6,11-DIHYDRO-11-ETHYL-6-METHYL-9-NITRO-5H-PYRIDO[2,3-B][1,5]BENZODIAZEPIN-5-ONE | C15 H14 N4 O3 | 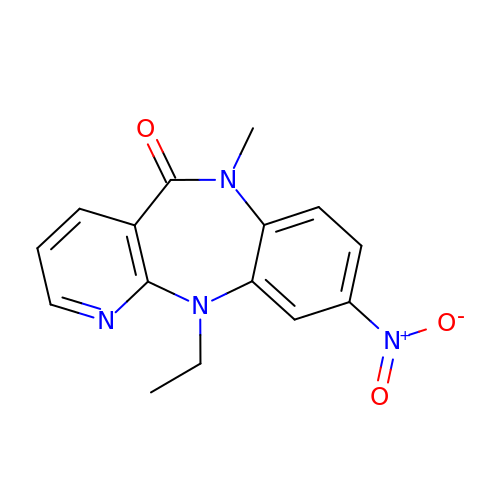YCFJZPGDTZVVSM-UHFFFAOYSA-N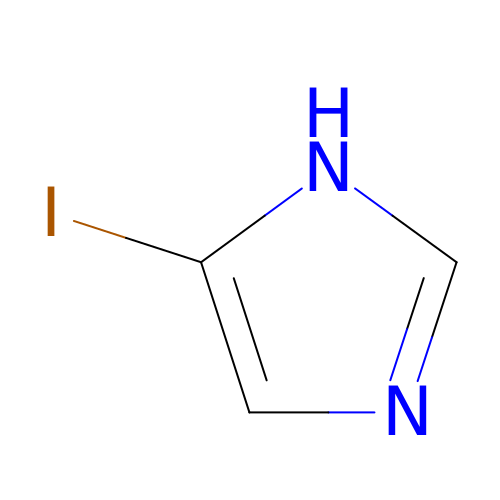5-iodo-1H-imidazole | C3 H3 I N2 | BHCMXJKPZOPRNN-UHFFFAOYSA-N1-(3,4,5-trihydroxyphenyl)dodecan-1-one | C18 H28 O4 | 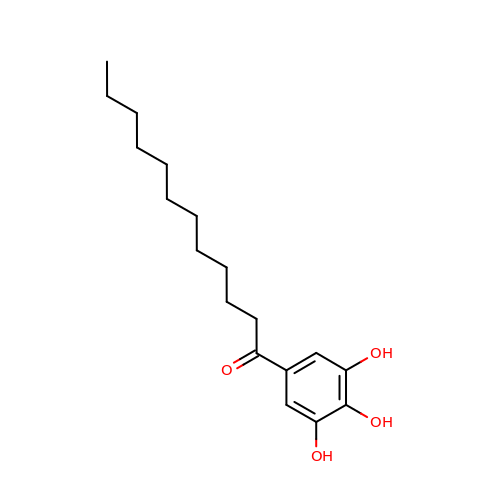TXMSPHFHTXABMF-UHFFFAOYSA-N N-{3-[5-(2-aminopyrimidin-4-yl)-2-tert-butyl-1,3-thiazol-4-yl]-2-fluorophenyl}thiophene-3-sulfonamide | C21 H20 F N5 O2 S3 | 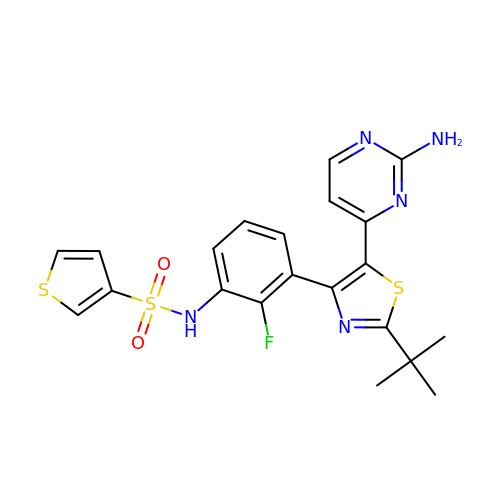CWSNFEIQSVSXSJ-UHFFFAOYSA-N> GSFTMDHYL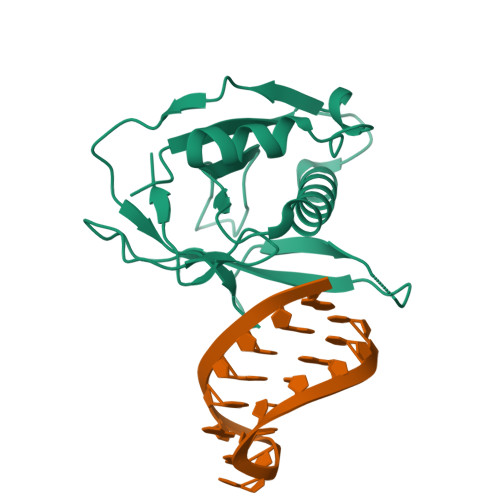DIRLRPDPEFPPAQLMSVLFGKLHQALVAQGGDRIGVSFPDLDESRSRLGERLRIHASADDLRALLARPWLEGLRDHLQFGEPAVVPHPTPYRQVSRVQAKSNPERLRRRLMRRHDLSEEEARKRIPDTVARALDLPFVTLRSQSTGQHFRLFIRHGPLQVTAEEGGFTCYGLSKGGFVPWF>[2x]MKFTVEREHLLKPLQQVSGPLGGRPTLPILGNLLLQVADGTLSLTGTDLEME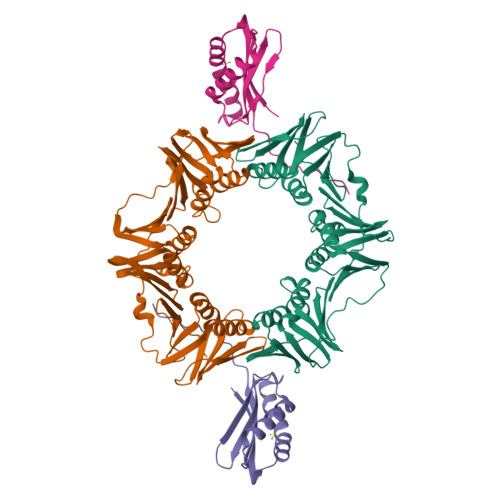MVARVALVQPHEPGATTVPARKFFDICRGLPEGAEIAVQLEGERMLVRSGRSRFSLSTLPAADFPNLDDWQSEVEFTLPQATMKRLIEATQFSMAHQDVRYYLNGMLFETEGEELRTVATDGHRLAVCSMPIGQSLPSHSVIVPRKGVIELMRMLDGGDNPLRVQIGSNNIRAHVGDFIFTSKLVDGRFPDYRRVLPKNPDKHLEAGCDLLKQAFARAAILSNEKFRGVRLYVSENQLKITANNPEQEEAEEILDVTYSGAEMEIGFNVSYVLDVLNALKCENVRMMLTDSVSSVQIEDAASQSAAYVVMPMRL;>HHHHHHVGVERTMAEDIHHWSECEAIIERLYPELERRLAKVKPDLLIARQGVKLKFDDFQQTTQEHVWPRLNKADLIATARKTWDERRGGRGVRLVGLHVTLLDPQMERQLVLGL[2x]>GPLGSMAEAFTREDYVFMAQLNENAERYDEMVETMRKISGMEGELSDKERNLLSVAYKNVIGPRRAAWRIVSSIEAKEKGRQKPNAKRIEQIRVYRQKIEKELSDICNDILKLLQEQFVPRSTNADAKVFYYKMQGDYYRYLAEYSSGEDKEKIAGSALNAYNSAFEISQQLPPTHPIRLGLALNFSVFYYEILASPDRACELARKAFDAAITDLDKLTEESYKDSTLIMQLLRDNLNLWVTDSAGDDNAEEK[4x]

Eukaryotic 14-3-3s are a family of dimeric highly conserved proteins (∼30 kDa) with pSer/pThr binding property. 14-3-3s bind to hundreds of client proteins thus affecting many cellular processes, including metabolism, signal transduction, cell cycle, differentiation, apoptosis, protein trafficking, transcription, stress responses and malignant transformation. Giardia posseses a single 14-3-3 isoform (g14-3-3) showing high sequence identity to the 14-3-3s of the epsilon subgroup. Interestingly, two post-translational modifications (PTMs) make g14-3-3 unique in the 14-3-3 protein family: constitutive phosphorylation and polyglycylation.

The structure of the g14-3-3 was determined at 3.2 Å resolution in the P32 space group and the asymmetric unit contained two functional dimers. Each g14-3-3 monomer displayed the typical 14-3-3 structural organization with nine antiparallel α-helices (A-I) arranged in a ‘U’ shaped fashion with a large central binding groove. The g14-3-3 N-terminal dimerization relies on residues largely conserved among the 14-3-3 family members involving, in this case, three salt bridges between Arg22 and Glu97, Asp9 and Lys82, and Glu25 and Lys93. Indeed, helix I of g14-3-3, compared with the human isoforms, is rotated of about 180° around helix H implying a substantial rearrangement of the loop connecting helices H and I (HI loop). As consequence of the helix I rearrangement, the g14-3-3 structure showed a fully open “extended” conformation of the C-terminal region, supporting the notion that the g14-3-3 region encompassing helices G and I possesses a degree of flexibility allowing the binding groove to change from a “closed” to an “open” conformation and thus accommodating different types of peptides. A possible consequence of such exposure of hydrophobic residues is the observed domain swapping occurring between the C-terminus of two g14-3-3 monomers, each belonging to a different dimer, in which helix I' from a monomer interacts with helices F and H from the monomer of the neighboring dimer. Domain swapping entails a dimerization event at the protein C-terminus with the formation of a four-helix bundle between two adjacent g14-3-3 dimers, leading to the assemblage of protein filaments. The overall g14-3-3 crystal packing resulted in stacks of endless parallel filaments, each layer being rotated 60° with respect to the previous one. The observed “extended” conformation of g14-3-3 with the large conformational change of helix I would disrupt the binding groove, which is indeed restored by domain swapping of helix I', indicating that the protein assemblies can retain phosphopeptide binding properties even in the case of C-terminal dimerization. The solved structure of g14-3-3 is not phosphorylated and Thr214 is buried at the C-terminal interface and its side chain establishes a hydrogen bond with Thr222.> GPLGSMTTKQTVSLFIWLPESKQKTLFISTKNHTQFELNNIIFDVTLSTELPDKEPNAIITKRTHPVGKMADEMRKYEKDHPKVLFLESSAIHDMMSSREEINALLIKNNIPIPNSFSVKSKEEVIQLLQSKQLILPFIVKPENAQGTFNAHQMKIVLEQEGIDDIHFPCLCQHYINHNNKIVKVFCIGNTLKWQTRTSLPNVHRCGIKSVDFNNQHLEDILSWPEGVIDKQDIIENSANRFGSKILEDPILLNLTSEAEMRDLAYKVRCALGVQLCGIDFIKENEQGNPLVVDVNVFP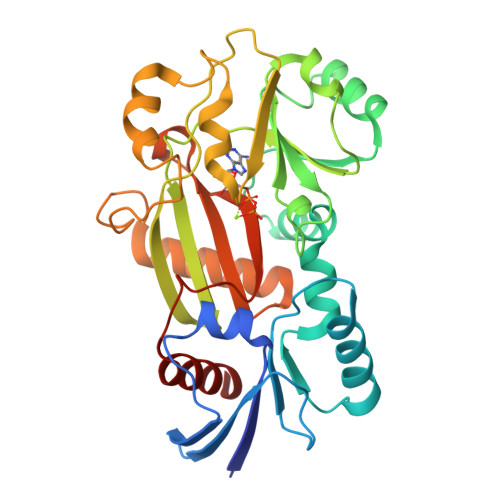SYGGKVDFDWFVEKVALCYTEVAKI>[2x]APSHPIFHRGEFSVCDSVSVWVADKTTATDIKGKEVMVLGEVNINNSVFKQYFF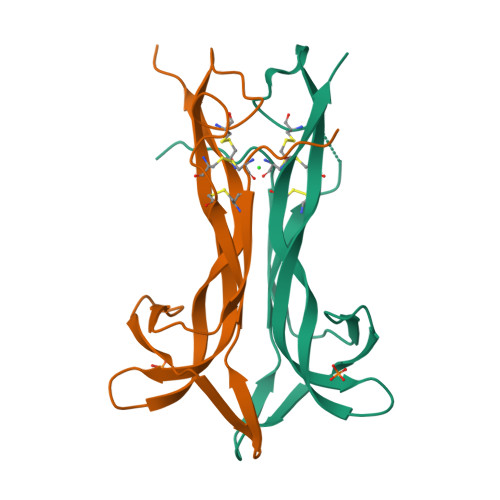ETKCRDPNPVASGCRGIDSKHWNSYCTTTHTFVKALTMDGKQAAWRFIRIDTACVCVLSKKAS>NLKPVDAMQCFDCHTQIEDMHTVGKHATVNCVHCHDATEHVETASSRRMGERPVTRMDLEACATCHTAQFNSFVEVRHESHPRLEKATPTSRSPMFDKLIAGHGFAFEHAEPRSHAFMLVDHFVVDRAYGGRFQFKNWQKVTDGMGAVRGAWTVLTDADPESSDQRR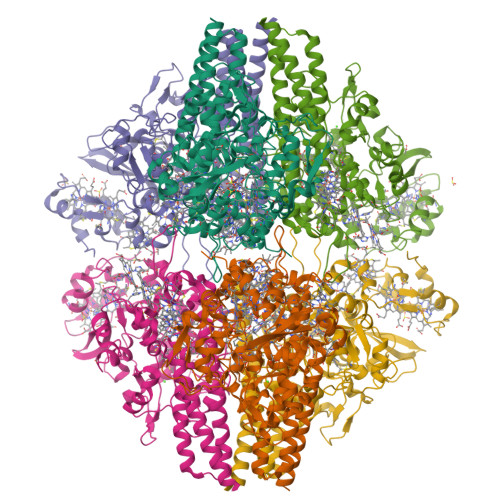FLSQTATAANPVCLNCKTQDHILDWAYMGDEHEAAKWSRTSEVVEFARDLNHPLNCFMCHDPHSAGPRVVRDGLINAVVDRGLGTYPHDPVKSEQQGMTKVTFQRGREDFRAIGLLDTADSNVMCAQCHVEYNCNPGYQLSDGSRVGMDDRRANHFFWANVFDYKEAAQEIDFFDFRHATTGAALPKLQHPEAETFWGSVHERNGVACADCHMPKVQLENGKVYTSHSQRTPRDMMGQACLNCHAEWTEDQALYAIDYIKNYTHGKIVKSEYWLAKMIDLFPVAKRAGVSEDVLNQARELHYDAHLYWEWWTAENSVGFHNPDQARESLMTSISKSKEAVSLLNDAIDAQVASR[2x]>GPDDYVPSQIAVNTSTLPGVVIGPADAHTYPRVIGELAGTSNQYVFNGGAIALMRGKFTPALPKIGSITYTFHQGNSRDSSDFDIYDIGVSGLGIIIGMAGYWPATPLVPINSSGIYIDPVGANTNPNTYNGATASFGARLFVAFVATGRLPNGYITIPTRQLGTILLEAKRTSLNNKGLT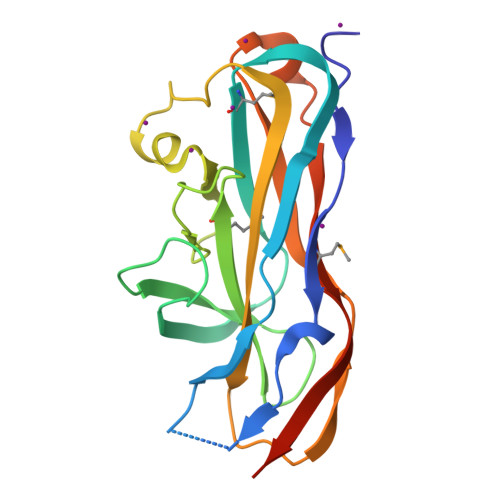APVMLNGGRIQVQSQTHHHHHH[2x]> F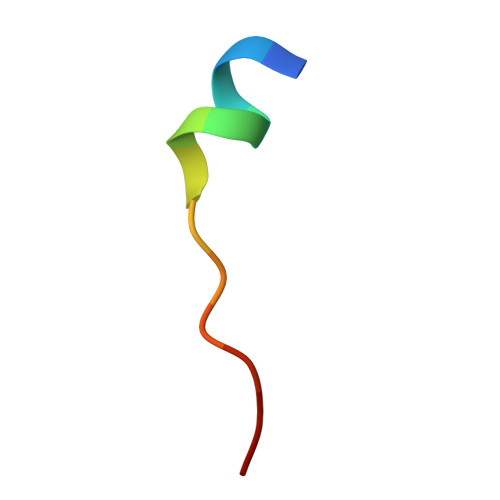TVLRKLNLVPIK>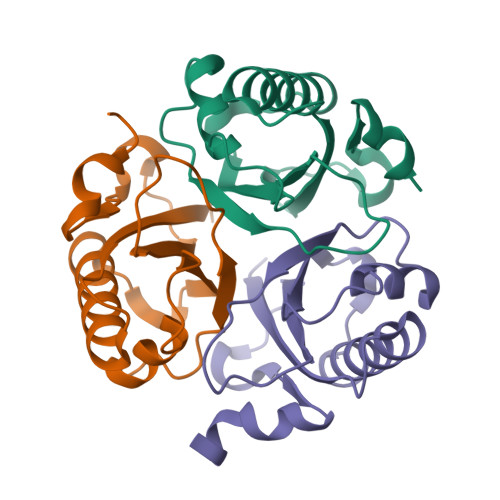MMFRGIRGATTVTEDTETEVLNKTKQLLEAIISRNEVDPERVVQILISATQDIHSVFPAKALRQFEGWTYVPVTCMQELDIHGGLKHCIRVLMTVQTDTKQEDVQHVYLEEAVTLRPDLQLTKNKELHHHHHH[6x]>[2x]MNAQAEEFKKYLETNGIKPKQFHKKELIFNQWDPQEYCIFLYDG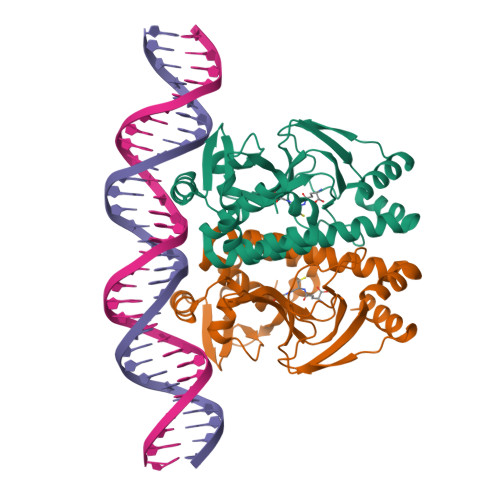ITKLTSISENGTIMNLQYYKGAFVIMSGFIDTETSVGYYNLEVISEQATAYVIKINELKELLSKNLTHFFYVFQTLQKQVSYSLAKFNDFSINGKLGSICGQLLILTYVYGKETPDGIKITLDNLTMQELGYSSGIAHSSAVSRIISKLKQEKVIVYKNSCFYVQNLDYLKRYAPKLDEWFYLACPATWGKLN> MRSLWSGVSGLQAHQVAMDVEGNNISNVNTTGFKYSRADFGTMFSQTVKIATAPTDGRGGSNPLQIGLGVSVSSTTRIHSQGSVQTTDKNTDVAINGDGFFMVSDDGGLTNYLTRSGDFKLDAYGNFVNNAGFVVQGWNINWDDQTIDSSRTPQNIFIDPGMHIPAAKSTEVAIKANLNSGLNIGTSSRNLYALDSVHGWNTKTQRAEDENDTGTTQFYTTSKNSVEVTEKGVDAGALFNANGTGLNLRDGQGIWVSYADAKFTTDRANGANVFDPNLTVAQQNNVIFWGNKDIAVTLDINLNGVRIQNDNIRSLDEAIAYINTFTAPTDTRDGTGVKAVKKADGSGIEFVNNNADGTTDNMKNIDLTVNVGNSAGERNTINYNANTGVFSPQGGNLTTAQNDTDWIAGAAQAGQPQNVKVVTAHKYIYSSNPVTIPPMINPDGGPAFQPNNGNRPTD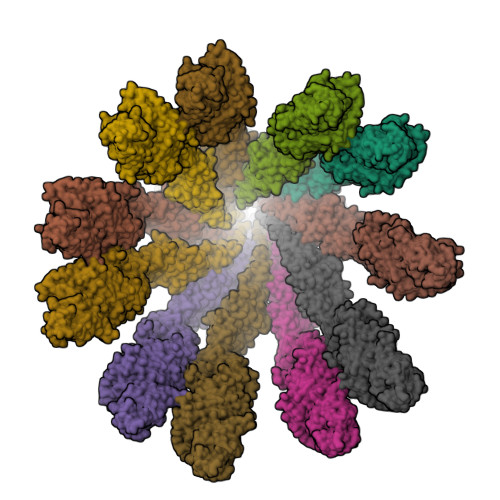PASANYWDAIQGSLKNTTERTFRTTEDLRELLQRDARYGVDYNGSGIIDNATPTFDANDINQAVKVVVTENGNFAISNANETSTIPANAGAGAGAATTNPKNMSFNITAYSNKQGTVSTNDAFTKIFKAFDGPLVIGNQIKESEQLKLSAFSAGLEIYDSLGSKHTLEVQFVKQSTTQDGGNEWQMIIRVPEPAEINTTGEGPTNIIVGTARFNNDGSLANYTPKTINFSPNNGAAPNQQIKLSFGTSGSNDGLVSSNSASTLTGQATDGYTSGNLKPDAIRVDDKGNILGEFTNGKTFAVAKIAMASVANNSGLEEIGGNLFKVTANSGNIVVGEAGTGGRGEMKTSALEMSNVDLSRSLTELIIIQRGYQANSKTISTSDQMLQTLIQLKQ>[5x]AMMPPRASIQQTADYL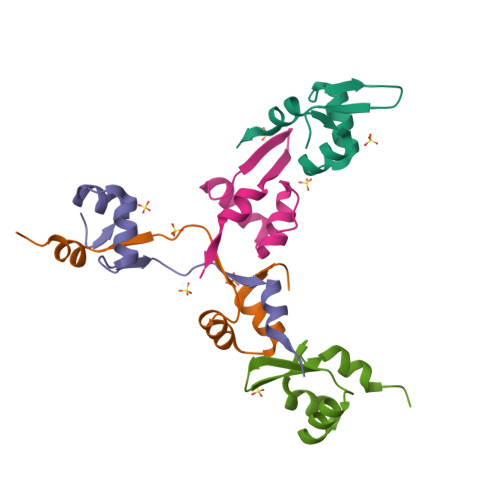GVSTKTVRNYIAAGKLKAVRLGPRLIRVERDSVEALMRPIGK> MAIYADNSYSIGNTPLVRLKHFGHNGNVVVKIEGRNPSYSVKCRIGANMVWQAEKDGTLTKGKEIVDPTSGNTGIALAYVAAARGYKITLTMPETMSLERKRLLCGLGVNLVLTEGAKGMKGAIAKAEEIVASDPSRYVMLKQFENPANPQIHRETTGPEIWKDTDGKVDVVVAGVGTGGSITGISRAIKLDFGKQITSVAVEPVESPVISQTLAGEEVKPGPHKIQGIGAGFIPKNLDLSIIDRVETVDSDTALATARRLMAEEGILAGISSGAAV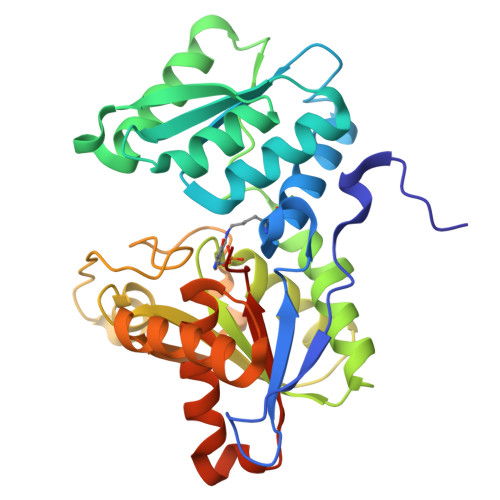AAADRLAKLPEFADKLIVVILPSASERYLSTALFEGIEG When a double helix is built with A·T Hoogsteen hydrogen bonds, an antiparallel double helix is formed, which has an appearance very similar to the standard B form of DNA. The main intrinsic change is the rotation of the glycosidic bond by 180°, so that the nucleoside conformation of adenine changes from anti to syn. A clear signature of the Hoogsteen form is the 2 Å shortening of the sugar C1’-C1’ distances across each base pair, which is clearly apparent in the structures determined by X-ray crystallography. In this paper we present a continuous Hoogsteen duplex with a non-alternating sequence, d(ATTAAT), which contains AA/TT base steps.

In the crystal the molecules are organized as columns of stacked duplexes, which are packed in a pseudo-hexagonal lattice. The electron density map of base pairs could be matched with the bases in the Hoogsteen conformation. Furthermore the average distance between the sugar C1’ atoms was short as expected. A significant feature of the present structure is the absence of any ligand in the minor groove. The present structure is stable by itself and does not require any additional ligands, but it is not clear why it crystallizes in the Hoogsteen form. In particular no trace of ethyl-aniline is apparent in the crystal structure, although it might help to stabilize the Hoogsteen form. Since the energetic difference between the Hoogsteen and W-C forms is rather small, it is likely that a combination of crystallization conditions, oligonucleotide length and sequence favored the Hoogsteen form in this particular case. The main conformational difference between the two conformations is found in the TA base step, which presents significantly different ωi twist values. Where ωi correspond to the twist angle between adjacent base pairs in the oligonucleotide and ωT correspond to the rotational setting angle of the virtual base step between stacked duplexes. In all Hoogsteen structures the value of ωT between neighbor duplexes is similar and close to 40°, only somewhat larger that the twist angle in the base steps inside the duplexes, as shown in Table 2.

>ATTAAT[5x]> MLTVLGRLLERNSIYVA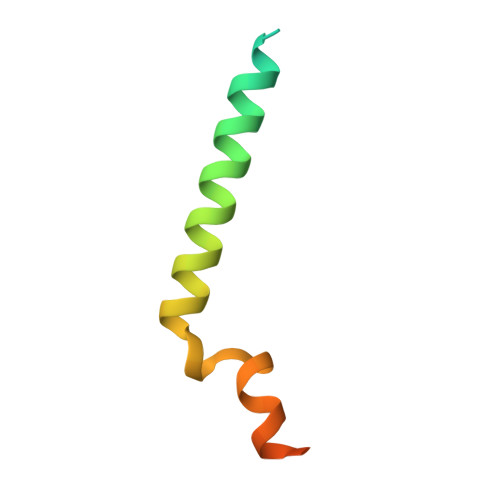TIFGGAFAFQGFFDVAVNKWWEEHNKAKLWKNVKGKFLEGEGEEEDDE>[2x]GYLDTSFYKQCRSILHVVMDLDRDGI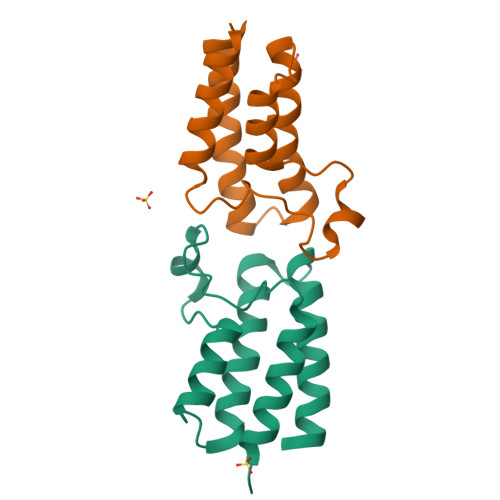FARDPSKLPDYRMIISHPMWWDLIKARLTRYEYTSPSAFINDMRLVVQNCYDYNREESPFSTLARRIEIAMEDLFVTELSL> ATHYSVADRWGNAVSVTYTINASYGSAASIDGAGFLLNNEMDDFSIKPGNPNLYGLVGGDANAIEANKRPLSSMSPTIVLKNNKVFLVVGSPGGSRIITTVLQVISNVIDYNMNISEAVSA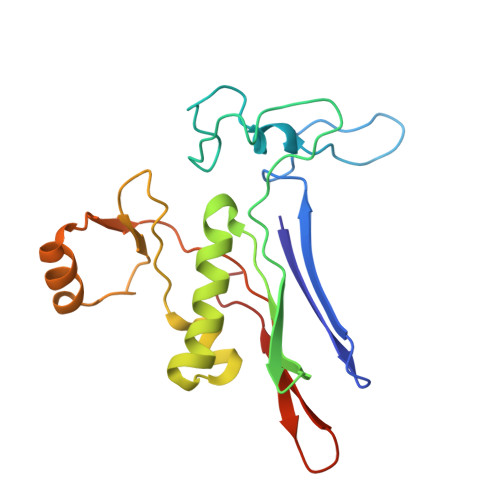PRFHMQWLPDELRIEKFGMPADVKDNLTKMGYQIVTKPVMGDVNAIQVLPKTKGSVFYGSTDPRKEF>GPGSELPQMVQQLNSPDQQELQSALWKLRNIASGGNEQIQAVIDAGALPALVQLLSSPNEQILSSALGALSNIASGGNEQIQAVIDAGALPALVQLLSSPNEQILQLALWALSNIASGGNEQIQAVIDAGALPALVQLLSSPNEQILQEALWALSNIASGGNEQIQAVIDAGALPALVQLLSSPNEQILQEALWALSNIASGGNEQIQAVIDAGALPALVQLLSSPNEQILQEALWALSNIASGGNEQKQAVKEAGALEKLEQLQ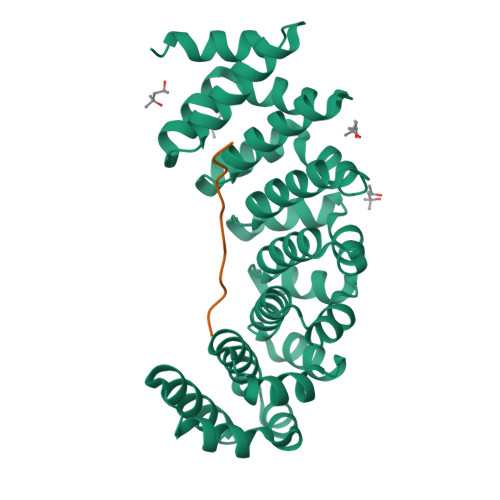SHENEKIQKEAQEALEKLQSH[2x];>[2x]KRKRKRKRKLSF>[4x]GPLGSAYAYLFKYIIIGDTGVGKSCLLLQFTDKRFQPVHDLTIGVEFGARMITIDGKQIKLQIWDTAGQESFRSITRSYYRGAAGALLVYDITRRDTFNHLTTWLEDARQHSN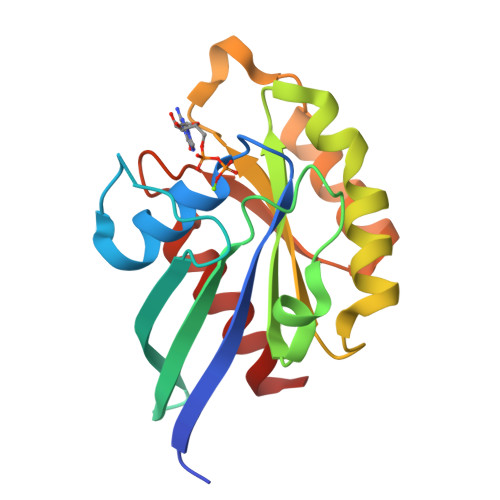SNMVIMLIGNKSDLESRREVKKEEGEAFAREHGLIFMETSAKTASNVEEAFINTAKEIYEK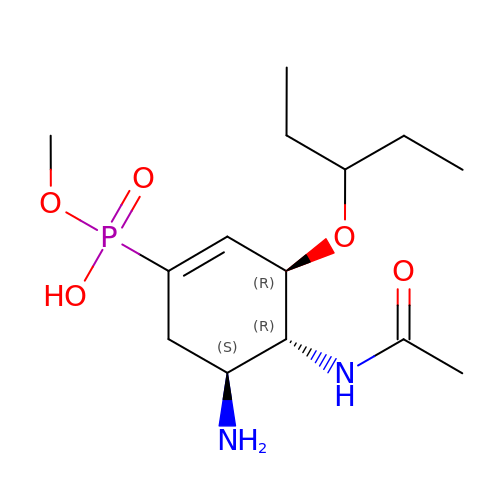[(3~{R},4~{R},5~{S})-4-acetamido-5-azanyl-3-pentan-3-yloxy-cyclohexen-1-yl]-methoxy-phosphinic acid | C14 H27 N2 O5 P | PYXVXICPPTUQQZ-BFHYXJOUSA-N> MGFIGNSLPMQAVYRVIESAASSKATVFITGESGTGKEVCAEAIHAASPRHDKPFIALNCAAIPKDLIESELFGHVKGAFTGASTERQGAVEMAHNGTLMLDELCEMDLDLQSKLLRFIQTGTYQKVGSSKMSSVDVRFVCATNRNPWEEVQEGRFREDLYYRLHVIPISLPPLRERGGDIIEIAHALLGLMSLEEGKSFSRFSEPVLRLFESYSWPGNVRELQNVIRNIVVLNTDDEVKLEMVPPPI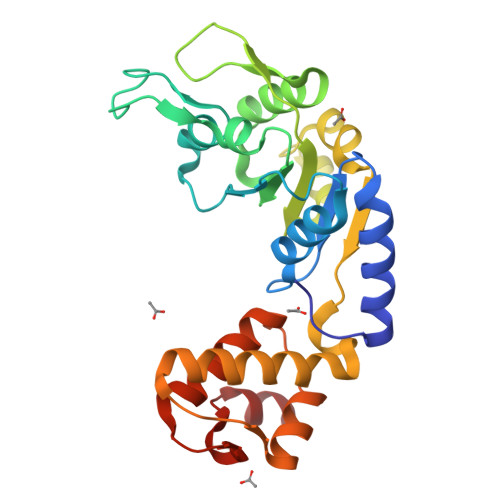LEHHH>MTSAEMTSPNNNSEHQAIAKMRTMIEGFDDISHGGLPIGRSTLVS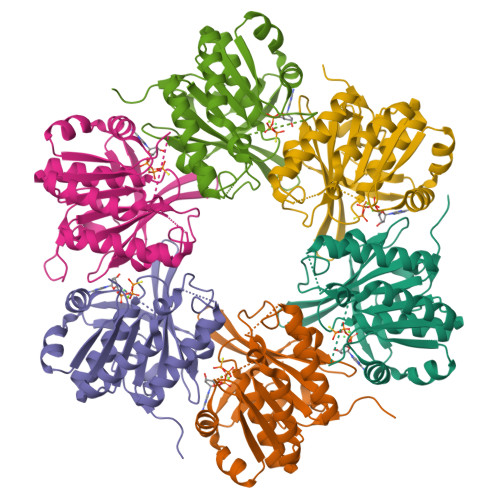GTSGTGKTLFSIQFLYNGIIEFDEPGVFVTFEETPQDIIKNARSFGWDLAKLVDEGKLFILDASPDPEGQEVVGGFDLSALIERINYAIQKYRARRVSIDPVTSVFQQYDASSVVRRELFRLVARLKQIGATTVMTTERIEEYGPIARYGVEEFVSDNVVILRNVLEGERRRRTLEILKLRGTSHMKGEYPFTITDHGINIFPLGAMR[6x]> AMTNNLYRLELERECVGC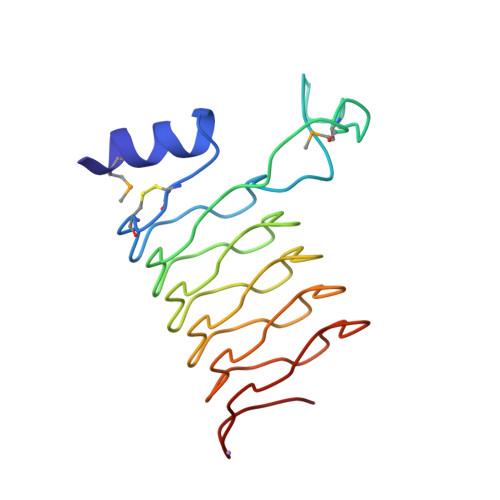NLEGVNLPRENFGLKYRIPRSSSPLVTTPFGMDKAKPVDLTRANLSNANLYQSDLSSIILENAILVETNLSETDLENAILIGANLQGANLENANLQGANLENANLRGAILTGVNLEETHLKGIETDKNTVWD(3~{S},4~{S})-4-(3,4-dimethylphenoxy)-1-prop-2-ynyl-piperidin-3-ol 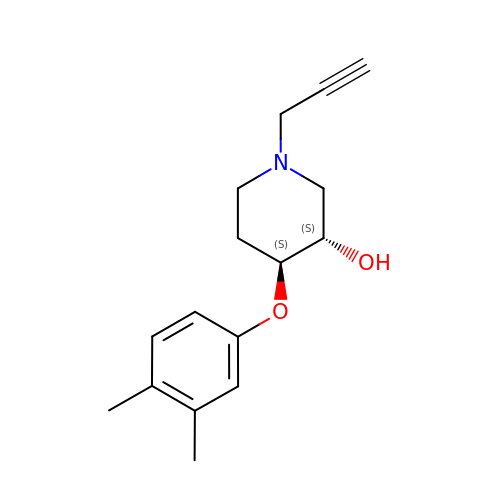| C16 H21 N O2 | DUHWBGRBPQCVNS-HOTGVXAUSA-N> GUGUGCCCGGCAUGGGUGCAGUCUAUAGGGUGAGAGUCCCGAACUGUGAAGGCAGAAGUAACAGUUAGCCUAACGCAACUGCGCCGUGGCGACAUGGCGUGGGAAGGAAGCGGACGGCAAACCUUCGGUCUGAGGAACACGAACUUCAUAUGAGGCUAGGUAUCAAUGGAUGAGUUUGCAUAACAAAACAAAGUCCUUUCUGCCAAAGUUGGUACAGAGUAAAUGAAGCAGAUUGAUGAAGGGAAAGACUGCAUUCUUACCCGGGGAGGUCUGGAAACAGAAGUCAGCAGAAGUCAUAGUACCCUGUUCGCAGGGGAAGGACGGAACAAGUAUGGCGUUCGCGCCUAAGCUUGAACCGCC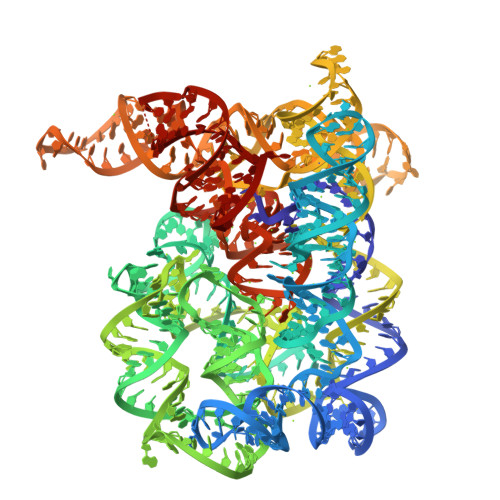GUAUACCGAACGGUACGUACGGUGGUGUGGCAGGGGCGCUUCGGCCCCCUAUGCCGAU>[2x]EVKLILYHWTHSFSSQKVRLVIAEKALKCEEHDVSLPLSEHNEPWFMRLNSTGEVPVLIHGENIICEATQIIDYLEQTFLDERTPRLMPDKESMYYPRVQRYRELLDSLPMDAYTHGCILHPELTVDSMIPAYATTRIRSQIGNTESELKKLAEENPDLQEAYIAKQKRLKSKLLDHDNVKYLKKILDELEKVLDQVETELQRRNEETPEEGQQPWLCGESFTLADVSLAVTLHRLKFLGFARRNWGNGKRPNLETYYERVLKRKTFNKVLGHVNNILIS

Charcot–Marie–Tooth disease (CMT) is the most common inherited peripheral polyneuropathy in humans, and its different subtypes are linked to mutations in dozens of different genes. Mutations in ganglioside‐induced differentiation‐associated protein 1 (GDAP1) cause two types of CMT, demyelinating CMT4A and axonal CMT2K. The GDAP1‐linked CMT genotypes are mainly missense point mutations. Structural analysis of GDAP1 indicates that CMT may arise from disruption of specific intra‐ and intermolecular interaction networks, leading to alterations in GDAP1 structure and stability, and, eventually, insufficient motor and sensory neuron function.

Here, we describe the biochemical and structural properties of the Finnish founding CMT2K mutation H123R and CMT2K‐linked R120W, both of which are autosomal dominant mutations. The disease variant proteins retain close to normal structure and solution behavior, but both present a significant decrease in thermal stability. Using GDAP1 variant crystal structures, we identify a side‐chain interaction network between helices ⍺3, ⍺6, and ⍺7, which is affected by CMT mutations, as well as a hinge in the long helix ⍺6, which is linked to structural flexibility.>[6x]GGPLGSMGNKVDKLAGVQELSVYEINERDRGSPVILPFGGKKDENGAHANSLGDLVPFSNKVYDGSLQRRLGITAGICTLISHNAEKKGDRYEAQYSFYFGDYGHISVQGPYIT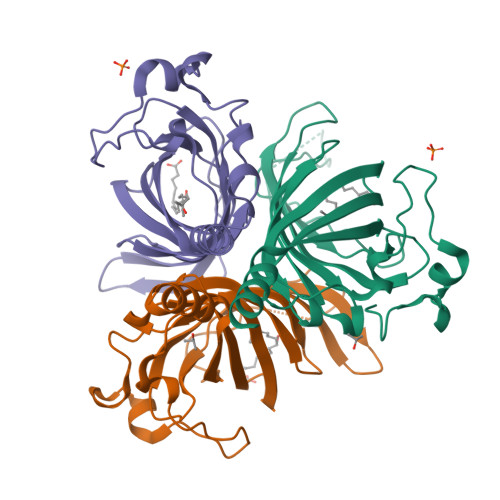YEDTELVVTGGTGIFAGCHGVAKLHQIIFPVKLFYTFYLQGIKKLPEELCASVVPPSPSAEPSEQAKKCHPSSVAPNFTN> MAMDQDKTVNWKVSLWVPPAHPLVPATKAWAEDIQKASGGSIRMTVFPSEQLGKAFDHYDMARDGIADVTYVNPGYQPGRFPIVSAGQLPFVFK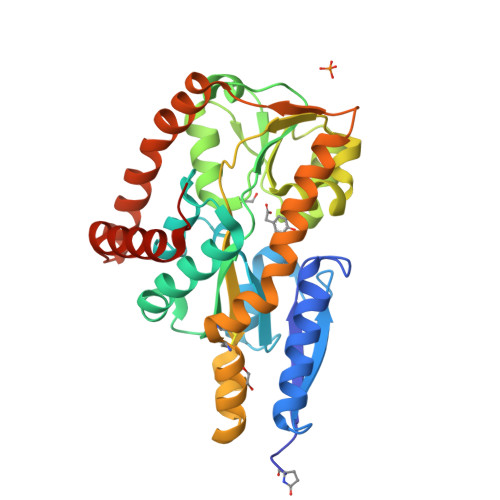DGKKGTLALNEWYHKYAPTEMKDTKLCFAFIHDPGALHGKKKVLLPSDLSGLKVRPAQSTIGEMVKLFGGTNVQASAPESRDALERGVADEITFPWGSVFLFGIDKVVKYHMDVPLYTTVFTYNIGLKAYNALSDAQKKIIDDHCTPEWASKVTDPWTDFEANGRVKMKALQDHEVYPLTDAQLAEWKKATKPLRDSWAEQVKKSGGDPAAVESDLQNALKKYDAGLHHHHHH> MSQTTTNPHVAVLAFPFSTHAAPLLAVVRRLAAAAPHAVFSFFSTSQSNASIFHDSMHTMQCNIKSYDISDGVPEGYVFAGRPQEDIELFTRAAPESFRQGMVMAVAETGRPVSCLVADAFIWFAADMAAEMGVAWLPFWTAGPNSLSTHVYIDEIREKIGVSGIQGREDELLNFIPGMSKVRFRDLQEGIVFGNLNSLFSRMLHRMGQVLPKATAVFINSFEELDDSLTNDLKSKLKTYLNIGPFNLITPPPVVPNTTGCLQWLKERKPTSVVYISFGTVTTPPPAEVVALSEALEASRVPFIWSLRDKARVHLPEGFLEKTRGYGMVVPWAPQA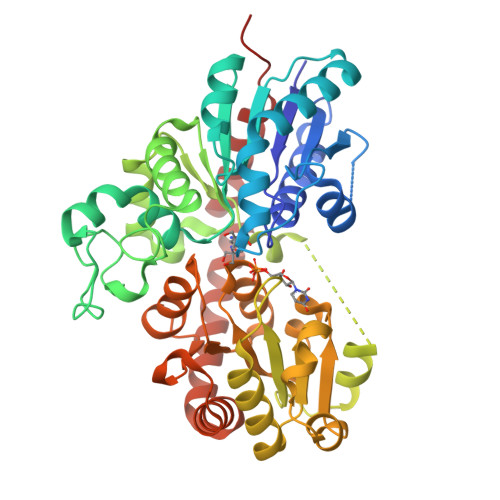EVLAHEAVGAFVTHCGWNSLWESVAGGVPLICRPFFGDQRLNGRMVEDVLEIGVRIEGGVFTKSGLMSCFDQILSQEKGKKLRENLRALRETADRAVGPKGSSTENFITLVDLVSKPKDV> MAHYPTRLKTRKTYSWVGRPLLDRKLHYQTYREMCVKTEGCSTEIHIQIGQFVLIEGDDDENPYVAKLLELFEDDSDPPPKKRARVQWFVRFCEVPACKRHLLGRKPGAQEIFWYDYPACDSNINAETIIGLVRVIPLAPKDVVPTNLKNEKTLFVKLSWNEKKFRPLSSELFAELNKPQESAAKCQKPVRAKSKSAESPSWTPAEHVAKRIESRHSASKSRQTPTHPLTPRARKRLELGNLGNPQMSQQTSCASLDSPGRIKRKVAFSEITSPSKRSQPDKLQTLSPALKAPEKTRETGLSYTEDDKKASPEHRIILRTRIAASKTIDIREERTLTPISGGQRSSVVPSVILKPENIKKRDAKEAKAQNEATSTPHRIRRKSSVLTMNRIRQQLRFLGNSKSDQEEKEILPAAEISDSSSDEEEASTPPLPRRAPRTVSRNLRSSLKSSLHTLTKVPKKSLKPRTPRCAAPQIRSRSLAAQEPASVLEEARLRLHVSAVPESLPCREQEFQDIYNFVESKLLDHTGGCMYISGVPGTGKTATVHEVIRCLQQAAQANDVPPFQYIEVNGMKLTEPHQVYVQILQKLTGQKATANHAAELLAKQFCTRGSPQETTVLLVDELDLLWTHKQDIMYNLFDWPTHKEARLVVLAIANTMDLPERIMMNRVSSRLGLTRMCFQPYTYSQLQQILRSRLKHLKAFEDDAIQLVARKVAALSGDARRCLDICRRATEICEFSQQKPDSPGLVTIAHSMEAVDEMFSSSYITAIKNSSVLEQSFLRAILAEFRRSGLEEATFQQIYSQHVALCRMEGLPYPTMSETMAVCSHLGSCRLLLVEPSRNDLLLRVRLNVSQDDVLYALKDE;> MSKPELKEDKMLEVHFVGDDDVLNHILDREGGAKLKKERAQLLVNPKKIIKKPEYDLEEDDQEVLKDQNYVEIMGRDVQESLKNGSATGGGNKVYSFQNRKHSEKMAKLASELAKTPQKSVSFSLKNDPEITINVPQSSKGHSASDKVQPKNNDKSEFLSTAPRSLRKRLIVPRSHSDSESEYSASNSEDDEGVAQEHEEDTNAVIFSQKIQAQNRVVSAPVGKETPSKRMKRDKTSDLVEEYFEAHSSSKVLTSDRTLQKLKRAKLDQQTLRNLLSKVSPSFSAELKQLNQQYEKLFHKWMLQLHLGFNIVLYGLGSKRDLLERFRTTMLQDSIHVVINGFFPGISVKSVLNSITEEVLDHMGTFRSILDQLDWIVNKFKEDSSLELFLLIHNLDSQMLRGEKSQQIIGQLSSLHNIYLIASIDHLNAPLMWDHAKQSLFNWLWYETTTYSPYTEETSYENSLLVKQSGSLPLSSLTHVLRSLTPNARGIFRLLIKYQLDNQDNPSYIGLSFQDFYQQCREAFLVNSDLTLRAQLTEFRDHKLIRTKKGTDGVEYLLIPVDNGTLTDFLEKEEEEA;> MATSSMSKGCFVFKPNSKKRKISLPIEDYFNKGKNEPEDSKLRFETYQLIWQQMKSENERLQEELNKNLFDNLIEFLQKSHSGFQKNSRDLGGQIKLREIPTAALVLGVNVTDHDLTFGSLTEALQNNVTPYVVSLQAKDCPDMKHFLQKLISQLMDCCVDIKSKEEESVHVTQRKTHYSMDSLSSWYMTVTQKTDPKMLSKKRTTSSQWQSPPVVVILKDMESFATKVLQDFIIISSQHLHEFPLILIFGIATSPIIIHRLLPHAVSSLLCIELFQSLSCKEHLTTVLDKLLLTTQFPFKINEKVLQVLTNIFLYHDFSVQNFIKGLQLSLLEHFYSQPLSVLCCNLPEAKRRINFLSNNQCENIRRLPSFRRYVEKQASEKQVALLTNERYLKEETQLLLENLHVYHMNYFLVLRCLHKFTSSLPKYPLGRQIRELYCTCLEKNIWDSEEYASVLQLLRMLAKDELMTILEKCFKVFKSYCENHLGSTAKRIEEFLAQFQSLDETKEEEDASGSQPKGLQKTDLYHLQKSLLEMKELRRSKKQTKFEVLRENVVNFIDCLVREYLLPPETQPLHEVVYFSAAHALREHLNAAPRIALHTALNNPYYYLKNEALKSEEGCIPNIAPDICIAYKLHLECSRLINLVDWSEAFATVVTAAEKMDANSATSEEMNEIIHARFIRAVSELELLGFIKPTKQKTDHVARLTWGGC;> MSSRKSKSNSLIHTECLSQVQRILRERFCRQSPHSNLFGVQVQYKHLSELLKRTALHGESNSVLIIGPRGSGKTMLINHALKELMEIEEVSENVLQVHLNGLLQINDKIALKEITRQLNLENVVGDKVFGSFAENLSFLLEALKKGDRTSSCPVIFILDEFDLFAHHKNQTLLYNLFDISQSAQTPIAVIGLTCRLDILELLEKRVKSRFSHRQIHLMNSFGFPQYVKIFKEQLSLPAEFPDKVFAEKWNENVQYLSEDRSVQEVLQKHFNISKNLRSLHMLLMLALNRVTASHPFMTAVDLMEASQLCSMDSKANIVHGLSVLEICLIIAMKHLNDIYEEEPFNFQMVYNEFQKFVQRKAHSVYNFEKPVVMKAFEHLQQLELIKPMERTSGNSEREYQLMKLLLDNTQIMNALQKYPNCPTDVRQWATSSLSWL;> MPHLENVVLCRESQVSILQSLFGERHHFSFPSIFIYGHTASGKTYVTQTLLKTLELPHVFVNCVECFTLRLLLEQILNKLNHLSSSEDGCSTEITCETFNDFVRLFKQVTTAENLKDQTVYIVLDKAEYLRDMEANLLPGFLRLQELADRNVTVLFLSEIVWEKFRPNTGCFEPFVLYFPDYSIGNLQKILSHDHPPEYSADFYAAYINILLGVFYTVCRDLKELRHLAVLNFPKYCEPVVKGEASERDTRKLWRNIEPHLKKAMQTVYLREISSSQWEKLQKDDTDPGQLKGLSAHTHVELPYYSKFILIAAYLASYNPARTDKRFFLKHHGKIKKTNFLKKHEKTSNHLLGPKPFPLDRLLAILYSIVDSRVAPTANIFSQITSLVTLQLLTLVGHDDQLDGPKYKCTVSLDFIRAIARTVNFDIIKYLYDFL

The origin recognition complex (ORC), composed of Orc1–6, is a highly conserved heterohexameric complex, which plays a critical role in recognizing origin DNA and promoting helicase loading. Each of the Orc1–5 subunits bears an AAA+ or AAA+-like domain and an α-helical winged-helix domain (WHD). Among Orc1–5, Orc1, Orc4, and Orc5 each contains a functional AAA+ domain for nucleotide binding; in contrast, Orc2 and Orc3 only contain a RecA-like subdomain with no predicted ATPase activities. Away from DNA, metazoan ORC resides in an autoinhibited conformation with a closed and constricted central channel to preclude DNA binding.

In order to acquire sufficient ORC samples with ORC1 incorporated, an additional high-salt incubation was applied to cell lysates to release ORC from chromatin. After this treatment, the amount of purified ORC subunits, especially ORC1, was substantially improved. While ORC1-WHD is located in a similar position as seen in previous ORC structures, ORC1-AAA+ is not as stable as that in the crystal structure of DmORC. In State I, in addition to its interactions with the AAA+ domains of ORC4 and ORC5 as seen in DmORC and ScORC structures, ORC1-WHD also engages with α3 of the HTH motif from ORC2-WHD through its β-hairpin motif. These interactions also induce noticeable conformational changes in other ORC subunits. Additional domain movements can also be observed on ORC2-AAA+ and ORC3-WHD, rendering a slight enlargement of the ORC ring. The weakened interface likely permits ORC2-WHD to sample more conformations. The interaction between ORC1-WHD and ORC2-WHD induces the transition from State I to State II, which is likely the first step of ORC activation for origin DNA binding.2-{bis[5-(trifluoromethyl)pyridin-2-yl]phosphoryl}-2-methyl-N-(2-{[2-(trifluoromethyl)phenyl]sulfanyl}ethyl)propanamide | C25 H21 F9 N3 O2 P S | 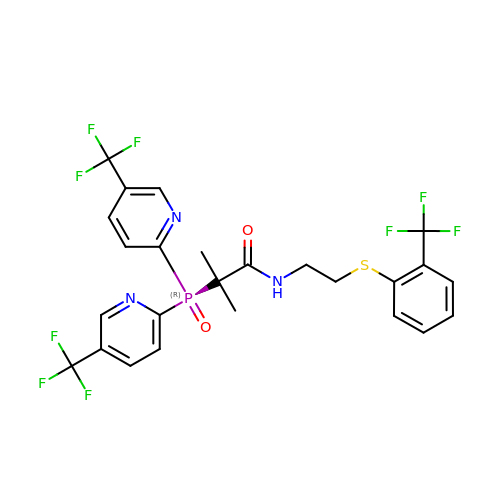YZQNSGLJZOYKHY-UHFFFAOYSA-N>[2x]MNPAAEAEFNILLATDSYKVTHYKQYPPNTSKVYSYFECREKKTENSKLRKVKYEETVFYGLQYILNKYLKGKVVTKEKIQEAKDVYKEHFQDDVFNEKGWNYILEKYDGHLPIEIKAVPEGFVIPRGNVLFTVENTDPECYWLTNWIETILVQSWYPITVATNSREQKKILAKYLLETSGNLDGLEYKLHDFGYRGVSSQETAGIGASAHLVNFKGTDTVAGLALIKKYYGTKDPVPGYSVPAAEHSTITAWGKDHEKDAFEHIVTQFSSVPVSVVSDSYDIYNACEKIWGEDLRHLIVSRSTQAPLIIRPDSGNPLDTVLKVLEILGKKFPVTENSKGYKLLPPYLRVIQGDGVDINTLQEIVEGMKQKMWSIENIAFGSGGGLLQKLTRDLLNCSFKCSYVVTNGLGINVFKDPVADPNKRSKKGRLSLHRTPAGNFVTLEEGKGDLEEYGQDLLHTVFKNGKVTKSYSFDEIRKNAQLNIELEAAHHLEHHHHHHHH

NAMPT functions as a homo-dimeric enzyme that catalyzes the rate limiting step in the primary salvage pathway for NAD synthesis, the transfer of a phosphoribosyl residue from 5-phosphoribosyl-1-pyrophosphate (PRPP) to nicotinamide (NAM) to produce nicotinamide mononucleotide (NMN). Crystal structures of NAMPT in numerous ligand-bound forms have been reported. These structures consistently display a NAMPT homo-dimer with two essentially identical active sites at the dimer interface. Typical NAMPT inhibitors were found to occupy the portion of active site responsible for NAM binding and a tunnel-shaped cavity extending from the NAM binding site. Furthermore, we determine the crystal structures of six NAMPT mutants in the apo form and in complex with various inhibitors and present a definitive model to explain the differential effects of the mutations on various structural classes of NAMPT inhibitors.

GNE-618 is a novel small molecule that potently inhibits NAMPT activity and exhibits efficacy in xenograft models of cancer. H191 and G217 together with D219 and Y188 form one side of the tunnel wall surrounding the cavity commonly occupied by NAMPT inhibitors. This proximity suggests that these mutations could directly interfere with GNE-618 binding. The H191 imidazole ring forms a herringbone stacking interaction with the GNE-618 phenyl linker moiety. The same interaction is observed for other bi-aryl sulfone inhibitors. The stacking interaction defined the orientation of the inhibitor linker moiety inside the tunnel passage and oriented the inhibitor's terminal group to exit the tunnel. The optimal orientation of H191 imidazole ring is facilitated by hydrogen bond interactions with D219 and a water molecule (WAT), which in turn interacts with the main chain carbonyl of Y188.>[2x]GSRFHYDRNNIAVGADESVVKEAHREV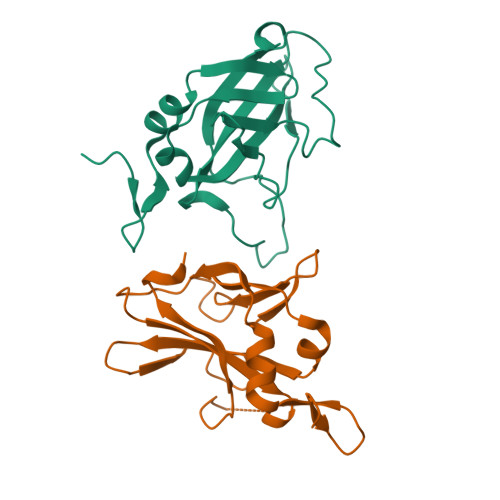INSSTEGLLLNIDKDIRKILSGYIVEIEDTEGLKEVINDRYDMLNISSLRQDGKTFIDFKKYNDKLPLYISNPNYKVNVYAVTKENTIINPSENGDTSTNGIKKILIFSKKGYEIG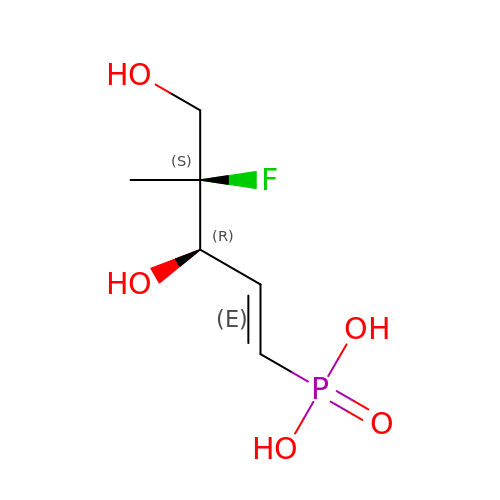[(1E,3R,4S)-4-FLUORO-3,5-DIHYDROXY-4-METHYLPENT-1-EN-1-YL]PHOSPHONIC ACID | C6 H12 F O5 P | FDKJTMXXMPIUAL-RITPCOANSA-N> GEIEFIESSKDAGFPVINTPSKTKLEPSVFHQVFEGNKEPAVLRSGDPRLKANFEEAIFSKYIGNVNTHVDEYMLEAVDHYAGQLATLDISTEPMKLEDAVYGTEGLEALDLTTSAGYPYVALGIKKRDILSKKTKDLTKLKECMDKYGLNLPMVTYVKDELRSIEKVAKGKSRLIEASSLNDSVAMRQTFGNLYKTFHLNPGVVTGSAVGCDPDLFWSKIPVMLDGHLIAFDYSGYDASLSPVWFACLKMILEKLGYTHKETNYIDYLCNSHHLYRDKHYFVRGGMPSGCSGTSIFNSMINNIIIRTLMLKVYKGIDLDQFRMIAYGDDVIASYPWPIDASLLAEAGKG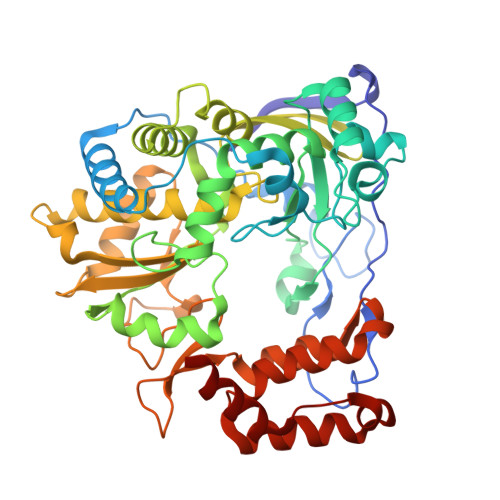YGLIMTPADKGECWNEVTWTNVTFLKRYFRADEQYPFLVHPVMPMKDIHESIRWTKDPKNTQDHVRSLCLLAWHNGEHEYEEFIRKIRSVPVGRCLTLPAFSTLRRKWLDSF> MENQLFIIGIGTGTDEYENFEETILKGVKRNELEGQIGPDILDNCCSDVCYFWGRSKETIYEKKIDKGDMVLFYVGKRISRNKVDLNQETAVYLGIICETVEISENDVSFLNDFWRKGENFRFLMFFKKKPEKLHHSINEINSKLGYNPDYFPIAGYVKPERMSGVYDILKNILKKRGILKESDSMNESAGHNIKEDYFRVDMLLNKKGQVILYGPPGTGKTWIARKYVVEETNEKTPGNKWEFITFHQSYSYEEFIEGFRPRTDNEEKIRYVVEDGIFKKIALRALVKGLFELEDATIGKDKIHRLYILLTKKEPLSPTEYEEYLRLKRYLWELVGGLPKDKLKNLTPKFYLIIDEINRGNISKIFGELITLLEKDKRLGGENQLIVRLPYSGEPFAVPPNLYIIGTMNTADRSIALLD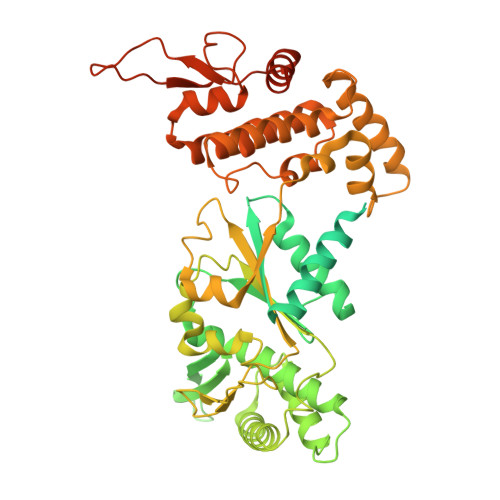VALRRRFAFIEVEPRPEFLEKENLKKIREKKLKTEDRKRLNEKLNELFSKLGNDNYFLKTLLEKINVRITVVKDRDHRIGHSYFLNVETVEDLHHVWYYEVLPLLMEYFYNDWETIKWVLNEKGKEHGNVFFEKLRLTGPNGEEAYQLKVLEGDAFIGALKRIISKNTPSQEGGATTNEENSPENTQSQTEGD>[10x]SMGKVNVAKLRYMSRDDFRVLTAVEMGMKNHEIVPGSLIASIASLKHGGCNKVLRELVKHKLIAWERTKTVQGYRLTNAGYDYLALKTLSSRQVVESVGNQMGVGKESDIYIVANEEGQQFALKLHRLGRTSFRNLKNKRDYHKYRHNVSWLYLSRLS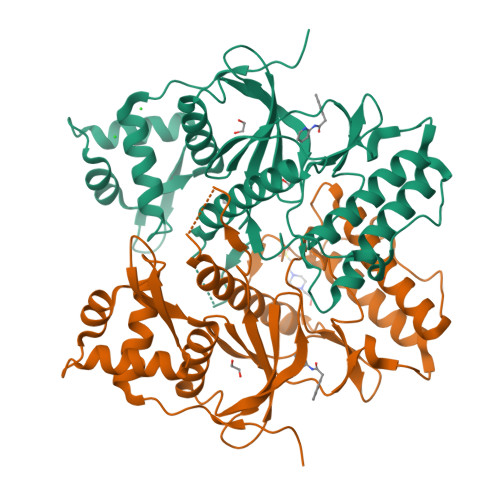AMKEFAYMKALYERKFPVPKPIDYNRHAVVMELINGYPLCQIHHVEDPASVYDEAMELIVKLANHGLIHGDFNEFNLILDESDHITMIDFPQMVSTSHPNAEWYFDRDVKCIKDFFMKRFSYESELFPTFKDIRREDTLDVEVSASGYTKEMQADDELLHPLGPDDKNIETK2-AMINOFLUORENE | C13 H11 N 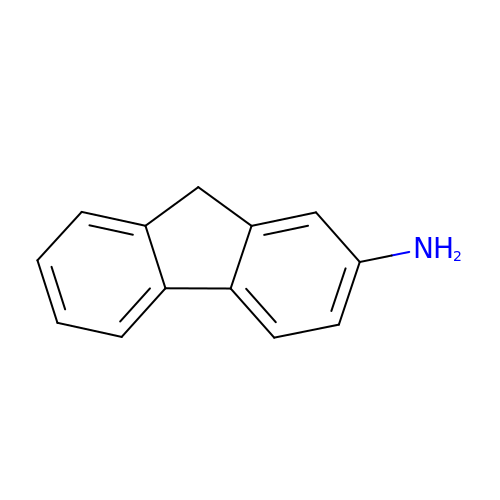| CFRFHWQYWJMEJN-UHFFFAOYSA-N> GIDPFTKEVVVNVDDDGVISLNFECDK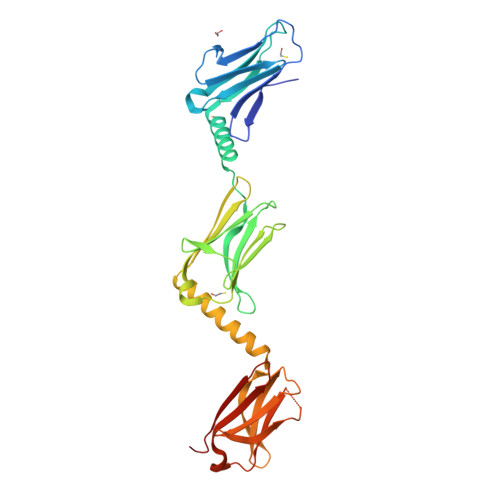MTPKSEFSWSKDYVSTEDSPRLEVESKGNKTKMTFKDLGMDDLGIYSCDVTDTDGIASSYLIDEEELKRLLALSHEHKFPTVPVKSELAVEILEKGQVRFWMQAEKLSGNAKVNYIFNEKEIFEGPKYKMHIDRNTGIIEMFMEKLQDEDEGTYTFQLQDGKATNHSTVVLVGDVFKKLQKEAEFQRQEWIRKQGPHFVEYLSWEVTGECNVLLKCKVANIKKETHIVWYKDEREISVDEKHDFKDGICTLLITEFSKKDAGIYEVILKDDRGKDKSRLKLVDEA>MKMDKKTIVWFRRDLRIEDNPALAAAAHEGSVFPVFIWCPEEEGQFYPGRASRWWMKQSLAHLSQSLKALGSDLTLIKTHNTISAILDCIRVTGATKVVFNHLYDPVSLVRDHTVKEKLVERGISVQSYNGDLLYEPWEIYCEKGKPFTSFNSYWKKCLDMSIESVMLPPPWRLMPITAAAEAIWACSIEELGLENEAEKPSNALLTRAWSPGWSNADKLLNEFIEKQLIDYAKNSKKVVGNSTSLLSPYLHFGEISVRHVFQCARMKQIIWARDKNSEGEESADLFLRGIGLREYSRYICFNFPFTHEQSLLSHLRFFPWDADVDKFKAWRQGRTGYPLVDAGMRELWATGWMHNRIRVIVSSFAVKFLLLPWKWGMKYFWDTLLDADLECDILGWQYISGSIPDGHELDRLDNPALQGAKYDPEGEYIRQWLPELARLPTEWIHHPWDAPLTVLKASGVELGTNYAKPIVDIDTARELLAKAISRTREAQIMIGAA[4x]

Cryptochromes (CRYs) are evolutionarily conserved photoreceptors that regulate numerous developmental networks including de-etiolation, photoperiodic control of flowering, root growth, plant height, organ size, stomatal opening, and stress responses. CRYs are comprised of two core domains: the highly conserved N-terminal photolyase homologous region (PHR) and the diversified carboxy-terminal extension (CCE). The chromophore, flavin adenine dinucleotide (FAD), is non-covalently bound to the C-terminal α subdomain of the PHR and plays a critical role in facilitating photoreduction. The CCE domain plays role in the regulation of CRYs by interacting with constitutive photomorphogenesis 1 (COP1) ubiquitin ligase as part of light signaling pathway.

Following extensive crystallization trials under full spectrum light conditions, we successfully determined the crystal structure of Arabidopsis CRY2-PHR in a tetrameric state (denoted AtCRY2-PHRtetamer). AtCRY2-PHRtetramer is comprised of four monomeric units (A, B, C, D) that are arranged as a ring-like structure with a central hollow cavity. The architecture within tetrameric AtCRY2-PHR is comprised of two different interfaces: a head to tail (H–T interface, monomers A–B) and head to head (H–H interface, monomers A–D) interaction between the monomers. In the AtCRY2-PHRtetramer, the interface (H–T) is assembled by the residues from α6, α12, α13, α18, α19, 310, L-24, L-26 and the second interface (H–H) is formed by the residues from α2, α10, α7, and L-11. The co-factor, FAD, adopts a typical U-shaped conformation and is buried inside the central core of C-terminal α domain, similar to the conformation reported in other structures of cryptochromes and photolysases. In the AtCRY2-PHRtetramer this connecting loop has two defined helices (α5 and α6) but it is largely disordered. Specifically, within AtCRY2-PHRtetramer H–T interface, the residue R208 (monomer A) forms ionic interactions with E428 (monomer B). Similarly, Q333 residue (monomer A) forms ionic interactions with E462 (monomer B), and bifurcated hydrogen bond interactions with T465 and N466 (monomer B). In AtCRY2-PHRinactive the α1 helix of BIC2 is inserted straight in the middle of the H-T interface and clearly clashes with the residues in α18, α19, and L-26, thus preventing or disrupting the H–T interface and oligomerization of AtCRY2.>MASWSHPQFEKGASLDSPTFGCTDSPVRRERGQKAVFCGLTSIVWLHRKMQDAFFLVVGSRTCAHLLQAAAGVMIFAEPRFGTAVLEEQDLAGLADAHKELDREVAKLLERRPDIRQLFLVGSCPSEVLKLDLDRAAERLSGLHAPHVRVYSYTGSGLDTTFTQGEDTCLAAMVPTLDTTEAAELIVVGALPDVVEDQCLSLLTQLGVGPVRMLPARRSDIEPAVGPNTRFILAQPFLGETTGALERRGAKRIAAPFPFGEEGTTLWLKAVADAYGVSAEKFEAVTAAPRARAKKAIAAHLETLTGKSLFMFPDSQLEIPLARFLARECGMKTTEIATPFLHKAIMAPDLALLPSNTALTEGQDLEAQLDRHEAINPDLTVCGLGLANPLEAKGHATKWAIELVFTPVHFYEQAGDLAGLFSRPLRRRALLNGGAA[2x];>[2x]MKLTLWTYEGPPHVGAMRVATAMKDLQLVLHGPQGCTYADLLFTMIERRNARPPVSFSTFEASHMGTDTAILLKDALAAAHARYKPQAMAVALTCTAELLQDDPNGISRALNLPVPVVPLELPSYSRKENYGADETFRALVRALAVPMERTPEVTCNLLGATALGFRHRDDVAEVTKLLATMGIKVNVCAPLGASPDDLRKLGQAHFNVLMYPETGESAARHLERACKQPFTKIVPIGVGATRDFLAEVSKITGLPVVTDESTLRQPWWSASVDSTYLTGKRVFIFGDGTHVIAAARIAAKEVGFEVVGMGCYNREMARPLRTAAAE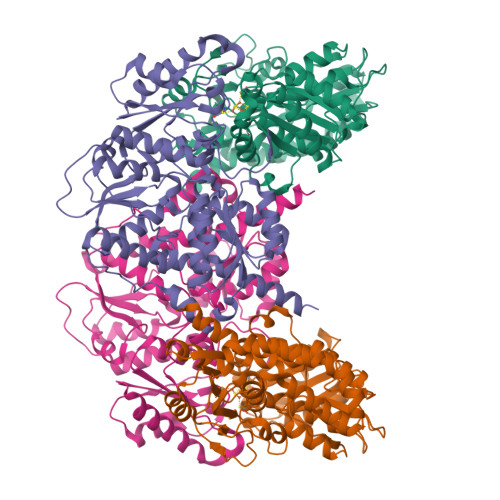YGLEALITDDYLEVEKAIEAAAPELILGTQMERNIAKKLGLPCAVISAPVHVQDFPARYAPQMGFEGANVLFDTWVHPLVMGLEEHLLTMFREDFEFHDAAGASHHGGKAVAREESPVAPADLAPAATSDTPAAPSPVVVTQASGEIRWMPEAERELRKIPFFVRGKAKRNTELYAAHKGVCDITVETLYEAKAHYAR> VFPSSVFVPDEWEVSREKITLLRELGQGSFGMVYEGNARDIIKGEAETRVAVKTVNESASLRERIEFLNEASVMKGFTCHHVVRLLGVVSKGQPTLVVMELMAHGDLKSYLRSLRPEAENNPGRPPPTLQEMIQMAAEIADGMAYLNAKKFVHRDLAARNCMVAHDFTVKIGDFGMTRDIYETAYYRKGGKGLLPVRWMAPESLKDGVFTTSSDMWSFGVVLWEITSLAEQPYQGLSNEQVLKFVMDGGYLDQPDNCPERVTDLMRMCWQFNPKMRPTFLEIVNLLKDDLHPSFPEVSF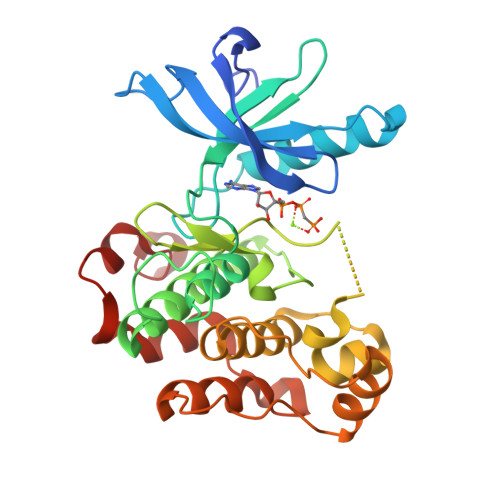FHSEENK>[2x]PSVYDAAAQLTADVKKDLRDSWKVIGSDKKGNGVALMTTLFADNQETIGYFKRLGNVS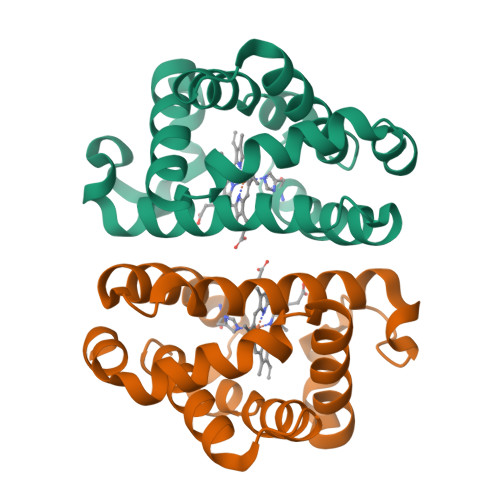QGMANDKLRGHSITLMYALQNFIDQLDNPDDLVCVVEKFAVNHITRKISAAEFGKINGPIKKVLASKNFGDKYANAWAKLVAVVQAAL>GPGSMAATIRYHEGDISAEDAARYKGAIAIDTETLGLVPRRDRLCVVQLSSGDGTADVIRIAAGQKQAPNLVHMLADPARQKIFHYGRFDIAVLFHTFGVTTTPVFCTKIASRLCRTYTDRHGLKDNLKEMLEVDISKAQQSSDWAAETLSPAQLEYAASDVLYLHALRDKLTARLIRDGRIEHADACFAFLPTRAKLDLLG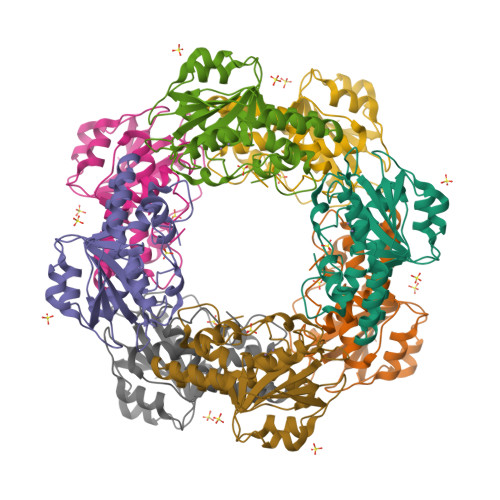WDETDIFAHS[2x]> SFTMSGGFELQPRDGGPRVALAPGETVIGRGPLLGITDKRVSRRHAILEVAGGQLRIKPIHTNPCFYQSSEKSQLLPLKPNLWCYLNPGDSFS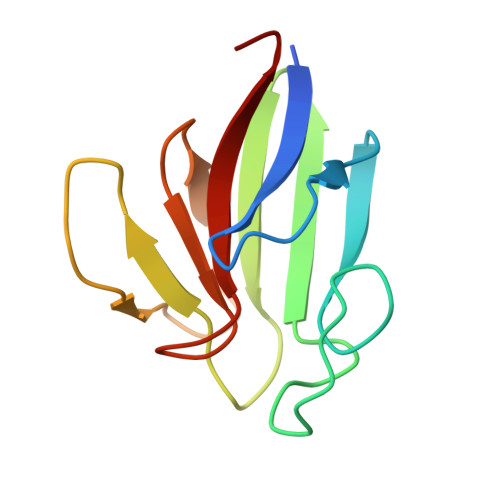LLVDKYIFRILSIPS> MAYLNRDQRREMILQAAMQIALAEGFTAMTVRRIATEAQTSTGQVHHHFSSASHLKAEAFLKLMEQLDEIEQTLQTTSQFQRLFILLGAENIDRLQPYLRLWNEAELLIEQDIEIQKAYNLAMQSWHQAIVQSIECGQKEGEFKNRSNSTDIAWRLIAFVCGLEGIYKLGLQGLAEEDFKRHT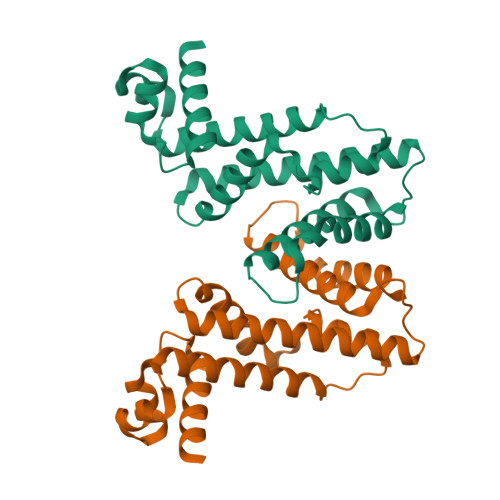EAIIRLELL>[8x]AMADLEQKVLEMEASTYDGVFIWKISDFARKRQEAVAGRIPAIFSPAFYTSRYGYKMCLRIYLNGDGTGRGTHLSLFFVVMKGPNDALLRWPFNQKVTLMLLDQNNREHV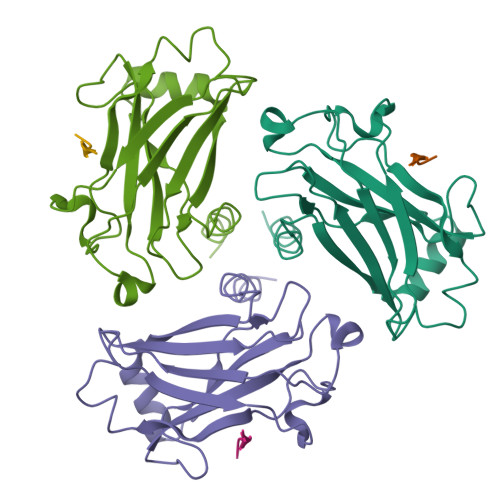IDAFRPDVTSSSFQRPVNDMNIASGCPLFCPVSKMEAKNSYVRDDAIFIKAIVDLTGL>MQIKQILSLIEEQQMSPDAGLELIRTYRKEQMGGGSPQQINDIVHRTITPLIEQQKIPGMAVAVIYQGKPYYFTWGYADIAKKQPVTQQTLFELGSVSKTFTGVLGGDAIARGEIKLSDPATKYWPELTAKQWNGITLLHLATYTAGGLPLQVPDEVKSSSDLLRFYQNWQPAWAPGTQRLYANSSIGLFGALAVKPSGLSFEQAMQTRVFQPLKLNHTWINVPPPEEKNYAWGYREGKAVHVSPGALDAEAYGVKSTIEDMARWVRSNMNPRDINDKTLQQGIQLAQSRYWQTGDMYQGLGWEMLDWPVNPDSIINGSGNKIALAAHPVKAITPPTPAVRASWVHKTGATGGFGSYVAFIPEKELGIVMLANKNYPNPARVAAAWQILNALQGGGSKNEDQEILF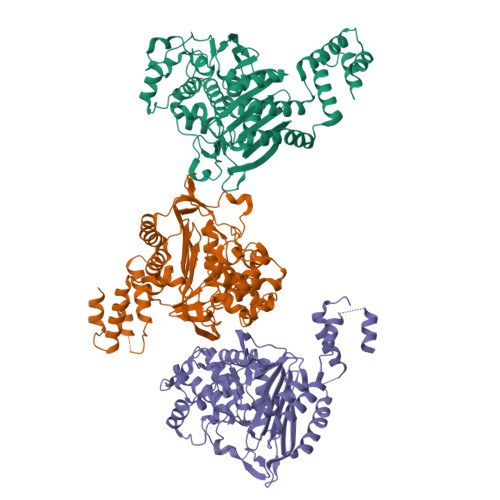LLEQLKNGELSADQVYQLLEGK[3x]>[4x]HMAEIYLAGGCFWGLEEYFSRISGVLETSVGYANGQVETTNYQLLKETDHAETVQVIYDEKEVSLREILLYYFRVIDPLSINQQGNDRGRQYRTGIYYQDEADLPAIYTVVQEQERMLGRKIAVEVEQLRHYILAEDYHQDYLRKNPSGYCHIDVTDADKPLIDAANYEKPSQEVLKASLSEESYRVTQEAATEAPFTNAYDQTFEEGIYVDITTGEPLFFAKDKFASGCGWPSFSRPLSKELIHYYKDLSHGMERIEVRSRSGSAHLGHVFTDGPRELGGLRYCINSASLRFVAKDEMEKAGYGYLLPYLNK;>SHMAEI[3x]

Oxidation of Met to methionine sulphoxide (Met-SO) damages the proteins and can alter protein function. However, these damaged proteins can be reversed by the repair enzymes, methionine sulphoxide reductases (Msr). Two distinct Msr enzymes have been classified for the reduction of Met-SO: MsrA reduces the S-form of Met-SO and MsrB reduces the R-form. However, enzymatic studies demonstrate that both the enzymes share a common catalytic mechanism based on sulphenic acid chemistry involving two (or three) cysteine residues.

In this study, we report the first crystal structure of MsrAB from S. pneumoniae (SpMsrAB). The monomeric structure of SpMsrAB has the overall dimensions of approximately 74.5 × 37.5 × 39.7 Å3 and consists of two major domains, MsrA (residues 1–158) and MsrB (residues 172–312), and a linker domain (residues 159–171). The linker, iloop, of SpMsrAB consists of 13 residues (residues 159–171) and, interestingly, contains one 310-helix and several hydrogen bonds to both the MsrA and MsrB domains that could restrict the positions of both domains. The asymmetric unit contains four molecules that show two conformations. Molecule A (Mol A) and molecule C (Mol C) are the same conformation (conformation 1) while molecule B (Mol B) and molecule D (Mol D) are the other conformation (conformation 2). Interestingly, Mol A contains an SHMAEI hexa-peptide and Mol B and Mol C have an SHMA peptide in their MsrB domains, but there appears no peptide bound in Mol D. This structure results from the crystal packing. Interestingly, as mentioned, our SpMsrAB structure reveals a complex between the active pocket of SpMsrB and the SHMAEI hexa-peptide, and is the first report of the structure of an MsrB complex with the product Met. The structure of the SpMsrB complex indicates that the catalytic Cys-284 faces the sulphur atom of the Met residue. We compared these two conformations and found that SpMsrA occurs in two dramatically distinct conformations relative to the centre of the iloop, while SpMsrB forms a complex with Met. Kinetic analysis revealed that the apparent Km value of SpMsrAB for Met-R-SO is 20-fold lower than that for Met-S-SO and the catalytic efficiency (kcat/Km) for the R-form is sevenfold higher than that for the S-form.>MAAQNEQRPERIKTTPYLEGDVLSSDSGPLLSVFALQEIMQKVRQVQADYMTATREVDFTVPDVQKILDDIKALAAEQVYKIVKVPSISFRHIVMQSRDRVLRVDTYYEEMSQVGDVITEDEPEKFYSTIIKKVRFIRGKGSFILHDIPTRDHRGMEVAEPEVLGVEFKNVLPVLTAEHRAMIQNALDGSIIENGNVATRDVDVFIGACSEPVYRIYNRLQGYIEAVQLQELRNSIGWLERLGHRKRITYSQEVLTDFRRQDTIWVLALQLPVNPQVVWDVPRSSIANLIMNIATCLPTGEYIAPNPRISSITLTQRITTTGPFAILTGSTPTAQQLNDVRKIYLALMFPGQIILDLKIDPGERMDPAVRMVAGVVGHLLFTAGGRFTNLTQNMARQLDIALNDYLLYMYNTRVQVNYGPTGEPLDFQIGRNQYDCNVFRADFATGTGYNGWATIDVEYREPAPYVHAQRYIRYCGIDSRELINPTTYGIGMTYHCYNEMLRMLVAAGKDSEAAYFRSMLPFHMVRFARINQIINEDLHSVFSLPDDMFNALLPDLIAGAHQNADPVVLDVSWISLWFAFNRSFEPTHRNEMLEVAPLIESVYASELSVMKVDMRHLSLMQRRFPDVLIQARPSHFWKAVLNDSPEAVKAVMNLSHSHNFINIRDMMRWVMLPSLQPSLKLALEEEAWAAANDFEDLMLTDQVYMHRDMLPEPRLDDIERFRQEGFYYTNMLEAPPEIDRVVQYTYEIARLQANMGQFRAALRRIMDDDDWVRFGGVLRTVRVKFYDARPPDDVLQGLPFSYDTNERGGLAYATIKYATETTIFYLIYNVEFSNTPDSLVLINPTYTMTKVFINKRIVERVRVGQILAVLNRRFVAYKGKMRIMDITQSLKMGTKLAAPTV[10x];> MVAITVQGAQLIKRVVERFYPGIAFNINEGACYIYKFSDHIRRIRMKHGTKYRRQAEEIIRNISLRKERLYGIPVLDEVEWKYVFDGQTFQSYAFEVYVNSILPWSELDPEEEFLRNYRVSREMTEVEKFIEFRAKNEMQIYGDIPIKVWCCFINELSAELKHVPLGMQVMADFVNRFDSPFHQGNRDLSNLEDFQVAYTTPLLFEMCCMESILEFNIKMRMREEEISALEFGDMKVDPVGLLREFFILCLPHPKKINNVLRAPYSWFVKMWGVGADPIVVLQSTAGDDRNSKDVFYDKFRTEPNRYKALFRSSFYNESRRMNEEKILEAVKYSQKLGSHDRRLPLFEKMLKTVYTTPFYPHKSSNMILASFLLSIQTITGYGRAWVKNVSTEFDKQLKPNPSNLVQDVSDLTREFFKQAYVEAKERREEIVKPEDLYTSMLRLARNTSSGFSTEIYVKKRFGPRLRDKDLIKINSRIKALVIFTKGHTVFTDEELHKKYNSVELYQTKGSRDVPIKATRTIYSINLSVLVPQLIVTLPLNEYFSRVGGITSPDYKKIGGKVIVGDLEATGSRVMDAADCFRNSADRDIFTIAIDYSEYDTHLTRHNFRTGMLQGIREAMAPYRDLRYEGYTLEQIIDFGYGEGRVANTLWNGKRRLFKTTFDAYIRLDESERDKGSFKVPKGVLPVSSVDVANRIAVDKGFDTLIAATDGSDLALIDTHLSGENSTLIANSMHNMAIGTLMQREVGREQPGVLTFLSEQYVGDDTLFYTKLHTTDTKVFDKVAASIFDTVAKCGHEASPSKTMMTPYSVEKTQTHAKQGCYVPQDRMMIISSERRKDIEDVQGYVRSQVQTMITKVSRGFCHDLAQLILMLKTTFIGAWKMKRTIKEDAMYRDRKFDSNDEDGFTLIQIRNPLALYVPIGWNGYGAHPAALNIVMTEEMYVDSIMISKLDEIMAPIRRIVHDIPPCWNETQGDKRGLISATKMSFFSKMARPAVQAALSDPQIINLVEELPLGEFSPGRISRTMMHSALLKESSARTLLSSGYELEYQKALNSWITQVSMRLGEESGVISTSYAKLFDVYFEGELDGAPHMFPDQNLSPQFYIQKMMIGPRVSSRVRNSYVDRIDVILRKDVVMRGFITANTILNVIEKLGTNHSVGDLVTVFTLMNIETRVAEELAEYMTSEKIRFDALKLLKKGIAGDEFTMSLNVATQDFIDTYLAYPYQLTKTEVDAISLYCTQMIMLRAALGLPKKKMKIVVTDDAKKRYKIRLQRFRTHVPKIKVLKKLIDPNRMTVRNLENQFV;> 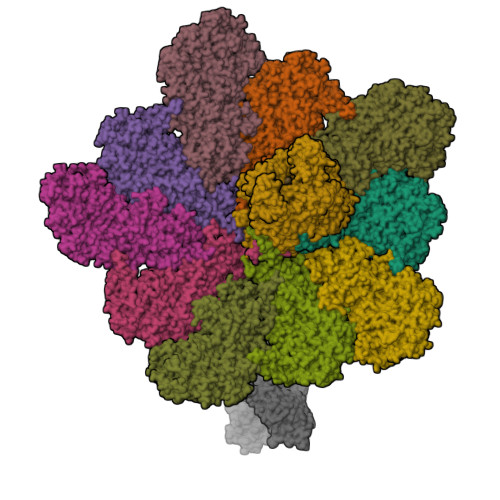MDELGIPVYKRGFPEHLLRGYEFIIDVGTKIESVGGRHDVTKIPEMNAYDIKQESIRTALWYNPIRNDGFVLPRVLDITLRGYDERRAVVESTRHKSFHTNDQWVQWMMKDSMDAQPLKVGLDDQSRNVAHSLHNCVVKIDSKKADTMSYHVEPIEDASKGCLHTRTMMWNHLVRIETFHAAQEVAYTLKPTYDIVVHAERRDRSQPFRPGDQTLINFGRGQKVTMNHNSYDKMVEGLAHLVIRGKIPEVIRDDIASLDEICNRWIQSRHDPGEIKAYELCKILSTIGRKVLDREKEPEDEASLSIRFQEAIDNKFRQHDPERLKIFEHRNQRRDEDRFYILLMIAASDTFNTRVWWSNPYPCLRGTLIASETKLGDVYSMMRSWYDWSVRPTYTPYEKTREQEKYIYGRVNLFDFVAEPGIKIVHWEYRLNHSTREITYAQGNPCDLYPEDDDVIVTKFDDVAYGQMINEMINGGWNQEQFKMHKILKSEGNVLTIDFEKDAKLTTNEGVTMPEYFNKWIIAPMFNAKLRIKHEEIAQRQSDDPMVKRTLSPITADPIELQRLTLARFYDIRPALRGQALSRQQAQSTYDEEISKRQDYAEILKRRGIVQIPKKPCPTVTAQYTLERYALFIISILQQHVVRDCDEEAVYEHPKADHELEIFGESIVDISQVIILAFDLIFERRRRVRDVYESRHIIARIRRMRGKERLNVIAEFFPTYGGLLNGLNSATVVQNIMYLNFLPLYFLVGDNMIYSHRQWSIPLLLYTHEVMVVPLEVGSYNDRCGLIAYLEYMVFFPSKAIRFSKLNEAQPKIAREMLKYYANTTVYDGGVNYNVVTTKQLLYETYLASLCGGISDGIVWYLPITHPNKCIVAIEVSDERVPASIRAGRIRLRFPLSARHLKGVVIIQIDEEGEFTVYSEGIVSHRVCKKNLLKYMCDIILLKFSGHVFGNDEMLTKLLNV>[4x]MSNCQYKIYPPLGIARVGNGPAIKPLSLSTPEVPWAHLYDTNVQYLVTQQELEQLLEEAFGGNVINEISQIKTKLDERKAEKFKQEEIETITGLLGLSHLVPQQQLSRSLDNLELKSTKDSDDIVQQIKGALLKVLSDHYLHAVKKQAQNFYIYKCDEQGNPVEKLKLTDGDKVTWRVEVANKKSFWYDY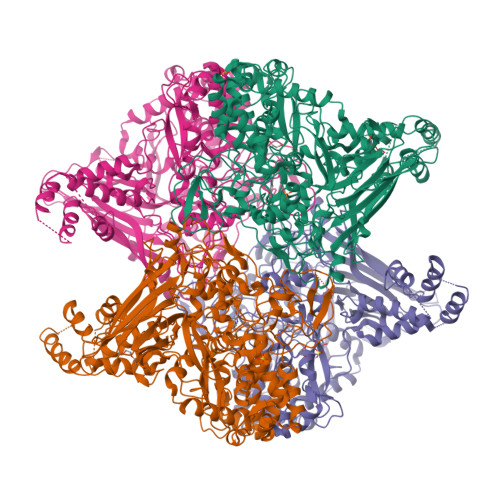NNALDLSLHTQGSGNLSKNVSKHRLAPAMTAKRRNPNVITNSLRKQLVISSQGSVSSDNNTQVPLRGKFPANEPDTNNRLSDLLNLQERHNVLQGSIECDNEGVLRFYAGNGISQALSPSSLNTDFADNSNWFDDICDGRVTAVVELKNGDTFEIQDEQSSAWVATTPPDYAPQIEPIVTMYDMVSGAALKEQDLDNLTTQFSDVFPILYRLYRMQWVNQADFTDNAVNTQIRELNSELGFAQLLDNSASAKSLREGIFNQFRNPLFDQDIDVDDPGQSSNEWVSNSRIIPSKDETNIAAKPATSSLKLPFYPNDGIDYPGSPVQWFAIPPFMYQHLQNWAAGDFSVTQVEKESANTIEELGLFYSEQFKNSPNSALLCARGALDALYGGGFCPGVELTWPMRHNLIYSQNDYVSSVTPEINLLGLREFRLKQDLQGLNSPNMYQDFGHVIAVDNVTASIDPNSDAAWLWRSTPGDLTKWMGIPWQSDAASCQAVYTPEDFPIPSWWAANLPVHVLPLARYNKFKDSQSADLPEINGMTHSIAQGMSEETFEHLRLEQFSQRLDWLHTADLGFVGYHAEGGYTNGLIQMVSQWKNMAMVMARPVENPGSSGIPNVVYVAYSQADKD> MGWSCIILFLVATATGVHSAPASSSTKKTQLQLEHLLLDLQMILNGINNYKNPKLTRMLTAKFAMPKKATELKHLQCLEEELKPLE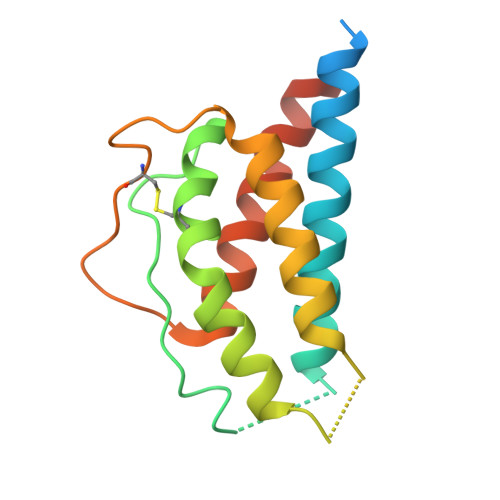EVLNGAQSKNFHLRPRDLISNINVIVLELKGSETTFMCEYADETATIVEFLNRWITFAQSIISTLTVDHHHHHH>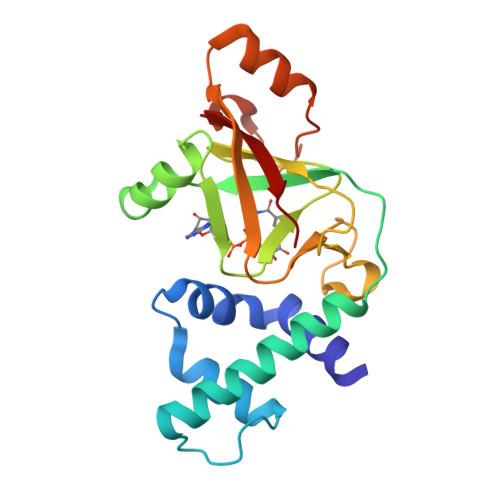 SKQIQALRYYSAQGYSVINKYLRGDDYPETQAKETLLSRDYLSTNEPSDEEFKNAMSVYINDIAEGLSSLPETDHRVVYRGLKLDKPALSDVLKEYTTIGNIIIDKAFMSTSPDKAWINDTILNIYLEKGHKGRILGDVAHFKGEAEMLFPPNTKLKIESIVNCGSQDFASQLSKLRLSDDATADTNRIKRIINMRVLNS>MYTSSMTYESLYTKYRDDSAILKTEDYAHWTLPTVYADPDLREGKRVNVRRDYQSVG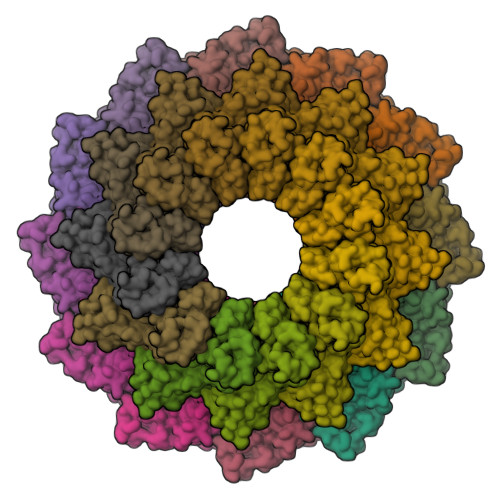AVYVNTLSAKLAQVLFPANQAFFRIDSTGDAAQLAEAMGAESADLANGLAELENTAFRRIFLKSSYHQLVHAMKLLIITGNVLLYRDSNTGNMHAYSIRQYSVLRDGGGKVLDMVLKERTVISELPVEARIKYRNRKQDDCICLYTRIKRERRAVGEVFVVTQQLEDGLMLDNLEVYPEAICPFIPAVWNLVTGETYGRGLVEDYAGDLAKLSALSEALALYEIEACRVLHMAKPGSQIDVDSMAERESGAWVAGDPNGVAAYEAGDYNKIIALTQEIQSIAARLAPAFMYAQNQRNAERVTAEEIRQNAEEAELALGGVYSVIADTLHIPLAHILCWEVNQQFINELLSNGLTLSVLTGVAALSRSTDVNKLIQAAQSLSVILPVFQNTPRVDPEKILDMVLTGFGINTKDLYRTEEQLQALQAAQAPVTPDLANVAGTINETGL[12x];>MELLDAVNTCLTALGEARVTSTDTRHPSVALILQTLATKQKLLLERGWWFNTQDEEMFPDLLGRIPYPAASISVESLDGYNIYSKRNNFLFNNTCNTMYFTGPVCIRVTYNLDFEDLPESVATVITYRAARAVYVGDLGNDASVQDLVLNEQQAMLLVEEQHMRNKKHSTRRRRPWGKYQNALSG[12x]> MIEPSVEEFPAENGPQLTPELAIANLQSSDLSLRYYAAWWLGKYRVKESAAVDALIAALEDEADRTELGGYPLRRNAARALGKLGNRKAVPGLINCLECPDFYVREAAAQSLEMLKDKTAAPALIKLLDGGVAQAVQVTGRPHLVQPYEAVLEALGAIGATDAIPLIQPFLEHPVSRVQCAAARAMYQLTQEPVYGELLVKVLAGNDLNLRRVALGDLGAIGYLAAAEAIANAKAENSFKLIALKGLLEHQMSAESNALSISDQAIRVMNLMDSLL;> MTNELINGVALADTPEKLVKAVQELALA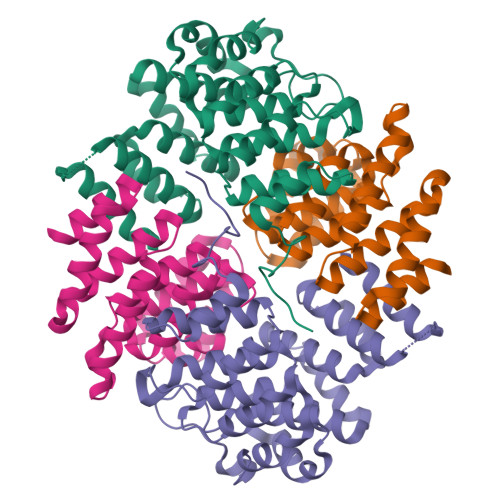KDVAAIPTLIAVFGYNNPTAAAIASTALVQLGEVAVPQLLTQIDDYNYGARAYSIRTLAAIADPRALDVLIDAAATDFAPSVRRAAAKGLGNLHWHKLEFPDNQTAPKKALETLLFISQDAEWSIRYAAIVGLQGLVNIPDLQQPIHTRLKEMLASDAEKAVRARILLAQSQLEHHHHHH> SVVIVGKISFCPKDVLGHGAEGTIVYRGMFDNRDVAVKRILPECFSFADREVQLLRESDEHPNVIRYFCTEKDRQFQYIAIELCAATLQEYVEQKDFAHLGLEPITLLQQTTSGLAHLHSLNIVHRDLKPHNILISMPNAHGKIKAMISDF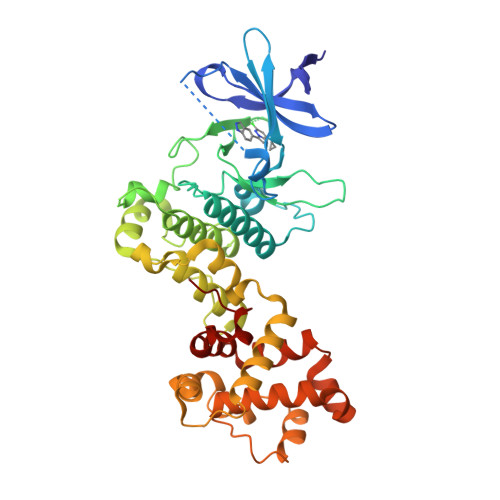GLCKKLAVGRHSFSRRSGVPGTEGWIAPEMLSEDCKENPTYTVDIFSAGCVFYYVISEGSHPFGKSLQRQANILLGACSLDCLHPEKHEDVIARELIEKMIAMDPQKRPSAKHVLKHPFFWSLEKQLQFFQDVSDRIEKESLDGPIVKQLERGGRAVVKMDWRENITVPLQTDLRKFRTYKGGSVRDLLRAMRNKKHHYRELPAEVRETLGSLPDDFVCYFTSRFPHLLAHTYRAMELCSHERLFQPYYFHE>[5x]MTKKVGIVDTTFARVDMASIAIKKLKELSPNIKIIRKTVPGIKDLPVACKKLLEEE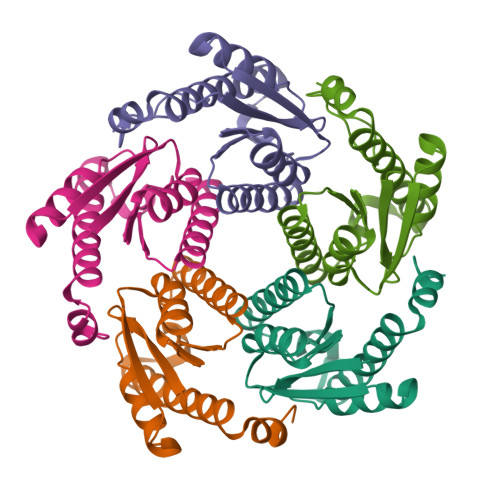GCDIVMALGMPGKAEKDKVCAHEASLGLMLAQLMTNKHIIEVFVHEDEAKDDKELDWLAKRRAEEHAENVYYLLFKPEYLTRMAGKGLRQGFEDAGPARE>MEKNVTQVKDTNNFPYNGVVSFKDATGFVIGKNTIITNKHVSKDYKVGDRITAHPNGDKGNGGIYKIKSISDYPGDEDISVMNIEEQAVERGPKGFNFNENVQAFNFAKDAKVDDKIKVIGYPLPAQNSFKQFESTGTIKRIKDNILNFD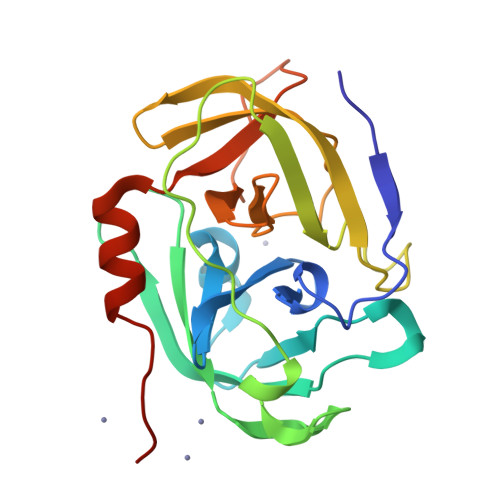AYIEPGNSGSPVLNSNNEVIGVVYGGIGKIGSEYNGAVYFTPQIKDFIQKHIEQHHHHHH[2x]>[4x]STPSIVIASAARTAVGSFNGAFANTPAHELGATVISAVLERAGVAAGEVNEVILGQVLPAGEGQNPARQAAMKAGVPQEATAWGMNQLCGSGLRAV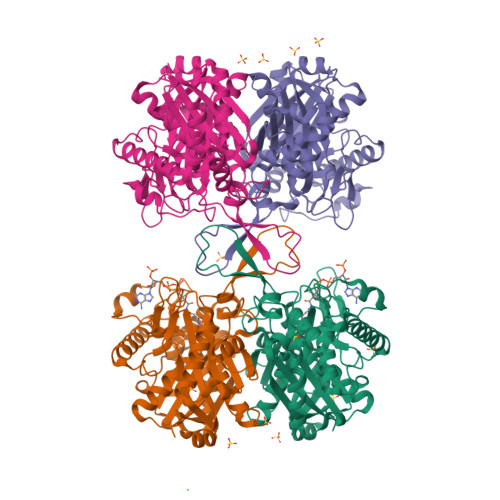ALGMQQIATGDASIIVAGGMESMSMAPHCAHLRGGVKMGDFKMIDTMIKDGLTDAFYGYHMGTTAENVAKQWQLSRDEQDAFAVASQNKAEAAQKDGRFKDEIVPFIVKGRKGDITVDADEYIRHGATLDSMAKLRPAFDKEGTVTAGNASGLNDGAAAALLMSEAEASRRGIQPLGRIVSWATVGVDPKVMGTGPIPASRKALERAGWKIGDLDLVEANEAFAAQACAVNKDLGWDPSIVNVNGGAIAIGNPIGASGARILNTLLFEMKRRGARKGLATLCIGGGMGVAMCIESL> MQSVNRKSNKGATANIDAQEPFSVLLMGIDTGDLGRTEQGRSDTTMVVTINPKENKSTMISLDRDILTDIVGNDTQDKLNHAYAFGGAEMAINTVQELLDIPIHHYVS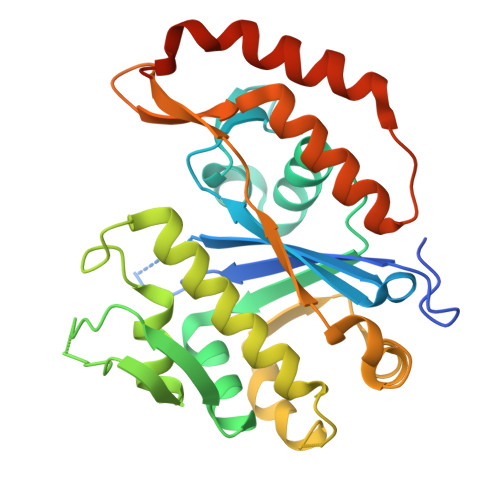INMKGLKDLIDAVGGIEVDNTIGEFTLDGITVPAGKIKLDGTTGLAYARMRHEDPEGDVGRQRRQREVVEKIVRKVMSFDGVSKYRKILDAVEANVKTDLTWDDMMDIQSKYLSAFKTIDSEQLQGYSATIDDIYYQVLDPNSLYKTQTTLRKQLGLKEHASEREKDLAFYNQFSYAVTDTALIGLEHHHHHH> MSVETPSALADSSPHTAPGSAGRSLELGAADIQDLESFEAGRGALPARAYLQSDAPRLSLNGEWQFRLSPGSRVAPDDGWQLGEALNGFESLPVPSSWPMHGHGAPAYTNVQFPFAVEPPHVPEANPIGDHLVVFEAGPEFFPHALLRFDGIESAGTVWLNGVELGTTRGSRLAHEFDVSGILEQGENTLAVRVAQFSAASYVEDQAMWWLPGIFRDVTLQARPAAGIDDVFVHAGYDHITGEGILKVEASRGGQAIDAVVRVPELALELAAGTEVRVPAVEPWSAEVPKLYEAAVSAAGESVALQIGFRSIAIEDAQFKVNGRRILLRGVNRHEHHPRLGRVVPRDVVEAELRLMKQHNINAIRTSHYPPHPQFLALADQLGFYVVLECDLETHGFESAGWAQNPSDDPQWEDALVDRMRRTVERDKNHASVVMWSLGNEAGTGRNLAAMSRWTKDRDPSRPIHYEGDWSSEHVDVYSRMYASQAETALIGQGIEPALNDAALDARRRAMPFVLCEYVHAMGNGPGGMSEYQALFEKYPRLMGGFVWEWLEHGITVSTADGVDHYGYGGDFGEEVHDGNFVTDGLVDADRRPRPGLLDFKKVIEPLRIDVARDWTGFTLRNGQDFADTSAFSFRYEVEADGGALDGGTVDVAPVAPQSETVVELPGSVAALAAGLSDGRPAVLTVRAVLGADSAWADAGHEVAWGQSVREPGAPVPPAPVEPVQVQDSELTLGPVVFSRATGMPTSIGGVPVEKLGLTLWWAP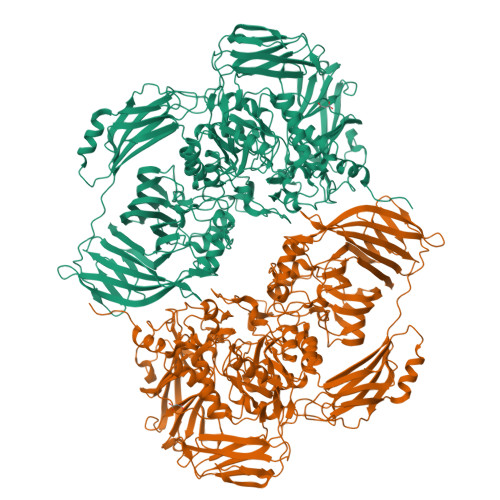TDNDLGREWGGADERPLATQWKDAGLNRLHTRLLGISANPGQDGGETLTVRTRVSAADKQYGVLVDYTWSTDGETVGLRTQVRRDGTWVNRGFEVEWARIGLEFVLGEETELVSWFGQGPHQSYPDTGQGARAGWFSLPLAKMDVEYVRPQECGARSGSRSAALQLGGRTLEICGDPFALTVRPYSQDVLDAAAHRPDLKADGRTYLYVDHALRGVGTAACGPGVLEQYRLKPRDADFILTLKVRS> MASTRGSGRPWSAKENKAFERALAVYDKDTPDRWANVARAVEGRTPEEVKKHYEILVEDIKYIESGKVPFPNYRTTGGNMKTDEKRFRNLK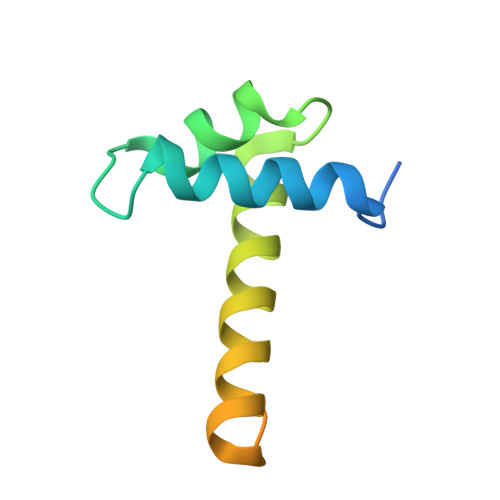IR>MTKENICIVFGGKSAEHEVSILTAQNVLNAIDKDKYHVDIIYITNDGDWRKQNNITAEIKSTDELHLENGEALEISQLLKESSSGQPYDAVFPLLHGPNGEDGTIQGLFEVLDVPYVGNGVLSAASSMDKLVMKQLFEHRGLPQLPYISFLRSEYEKYEHNILKLVNDKLNYPVFVKPANLGSSVGISKCNNEAELKEGIKEAFQFDRKLVIEQGVNAREIEVAVLGNDYPEATWPGEVVKDVAFYDYKSKYKDGKVQLQIPADLDEDVQLTLRNMALEAFKATDCSGLVRADFFVTEDNQIYINETNAMPGFTAFSMYPKLWENMGLSYPELITKLIELAKERHQ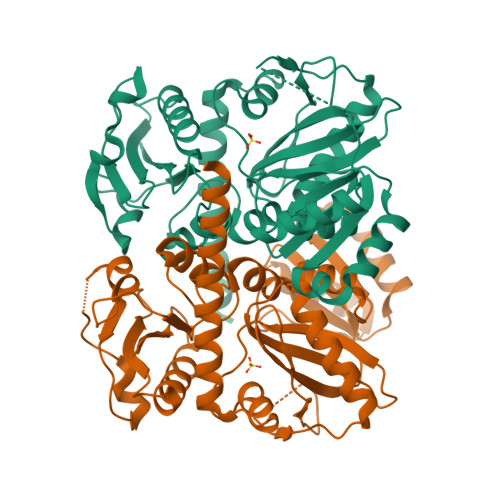DKQKNKYKIDRSHHHHHH[2x]> MKNFRLSEKEVKTLAKRIPTPFLVASLDKVEENYQFMRRHLPRAGVFYAMKANPTPEILSLLAGLGSHFDVASAGEMEILHELGVDGSQMIYANPVKDARGLKAAADYNVRRFTFDDPSEIDKMAKAVPGADVLVRIAVRNNKALVDLNTKFGAPVEEALDLLKAAQDAGLHAMGICFHVGSQSLSTAAYEEALLVARRLFDEAEEMGMHLTDLDIGGGFPVPDAKGLNVDLAAMMEAINKQIDRLFPDTAVWTEPGRYMCGTAVNLVTSVIGTKTRGEQPWYILDEG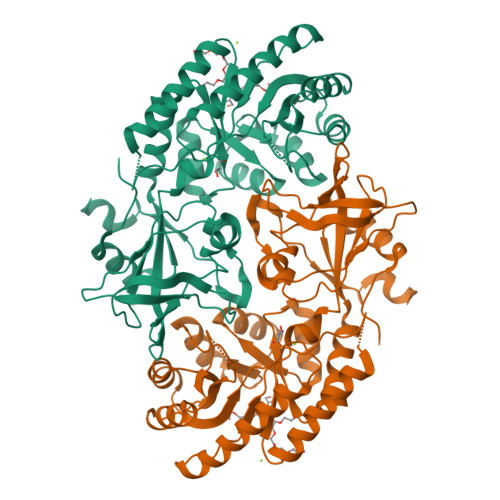IYGCFSGIMYDHWTYPLHCFGKGNKKPSTFGGPSCDGIDVLYRDFMAPELKIGDKVLVTEMGSYTSVSATRFNGFYLAPTIIFEDQPEYAARLTEDDDVKKKAAV> MRSGDAEIKGIKPKVIEEYSLSQGSGPSNDSWKSL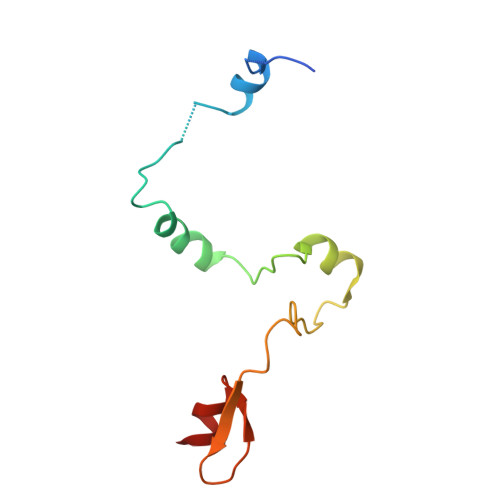MSSAKDTPLQYDHMNRESLKKYFNPNAQLIEDPLDKPIQYRVCEKCGKPLALTAIVDHLEN>SNSFEVSSLPDANGKNHITAVKGDAKIPVDKIELYMRGKASGDLDSLQAEYNSLKDARISSQKEFAKDPNNAKRMEVLEKQIHNIERSQDMARVLEQAGIVNTASNNSMIMDKLLDSAQGATSANRKTSVVVSGPNGNVRIYATWTILPDGTKRLSTVTGTFK[2x];>SNAMINVNSTAKDIEGLESYLANGYVEANSFNDPEDDALECLSNLLVKDSRGGLSFCKKILNSNNIDGVFIKGSALNFLLLSEQWSYAFEYLTSNADNITLAELEKALFYFYC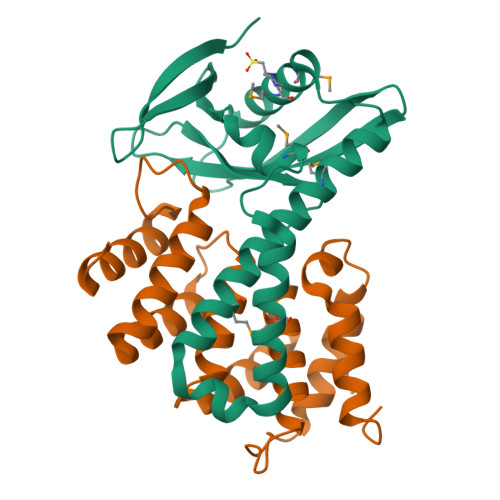AKNETDPYPVPEGLFKKLMKRYEELKNDPDAKFYHLHETYDDFSKAYPLNN[2x]>[4x]GPGSEFRQDKMREEGLQLVSMIREGEAAGACPEEIFSALQYSGTEV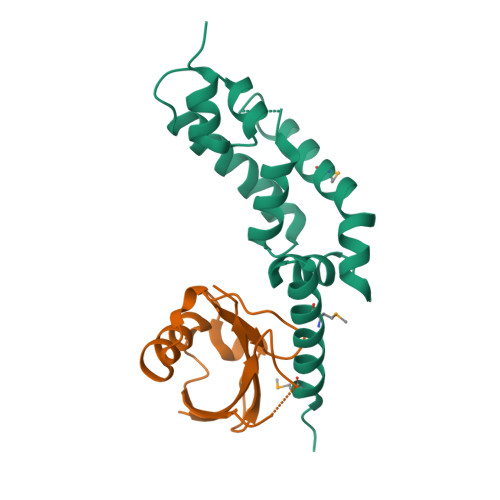PLQWLRSELPYVLEMVAELAGQQDPGLGAFSCQEARRAWLDRHGNLDEAVEECVRTRRRKVQELQSLGFGPEEGSLQALFQHGGDVSRALTELQRQRLEPFRQRLWDSGPEPTPSWDGPD;>[4x]GPGSSVQLQEACFPPGPIRLQVTLEDAASAASAASSAHVALQVHPHCTVAALQEQVFSELGFPPAVQRWVIGRCLCVPERSLASYGVRQDGDPAFLYLLSAPREAPAT>[2x]MKNLDINTFDNIEDIPLGSSEQDPYDFFTLSDRNVMNSDMKKNIVQWNSRYSYNQLKNKDSLIMFLVEIFRSLFVSNCIDKNIDNVLLSIEEMFIDHYYNPQHSRLKYLIDDVGIFFTKLPITKAFHTYNKKYRITKRLYAPPTFNEVRHILNLAQILSLEEGLDLLTFDADETLYPDGHDFNDE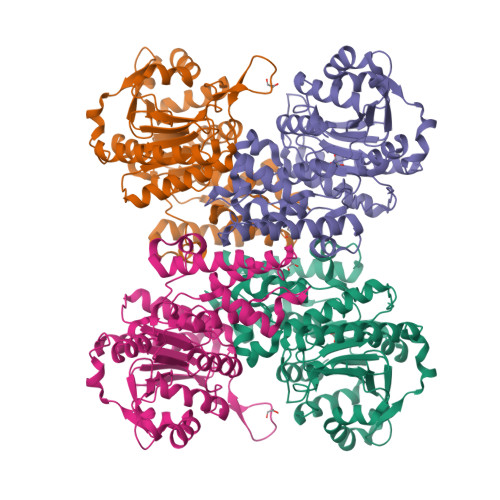VLASYISCLLKKMNIAIVTAASYNNDAEKYQKRLENLLKYFSKHNIKDGSYKNFYVMGGESNYLFKCNEEATLYSVPENEWRHYKKFVDYDTVQEILNISEKCLEKVIKDFGLCAQIQRKEKSIGLVPNKIPSLNIKNEQKNYMIKYEVLEEAVIRIKKEIIKNKITAPYCAFNGGQDLWVDVGNKAEGLLILQKLLKIQKKKCCHIGDQFLHSGNDFPTRFCSLTLWVSNPQETKACLKSIMHLN Recently, a shortened Dscam (sDscam) gene family with tandemly arrayed 5′ cassettes in Chelicerata species has been identified, which encodes ∼50–100 isoforms. Chelicerata sDscams could be classified into two subfamilies, sDscamα and sDscamβ, containing one and two variable Ig domains, respectively. Crystal structures and cell aggregation assays demonstrated that both α and β subfamilies of sDscam used Ig1 for the isoform-specific trans recognition in a hand-in-hand manner. Furthermore, the cis interactions were established by the three FNIII domains of sDscam, which assemble into a cross fold with a kink between FNIII2 and FNIII3.

The crystal structures of sDscam Ig1 from both M. martensii and L. polyphemus revealed a common assembly of antiparallel homodimer for both α and β subfamilies of sDscam. More interestingly, in some Ig1 crystal structures (M. martensii α1, α7, and L. polyphemus α7), the two protomers within a homodimer were related via a 2-fold symmetry axis, namely, these two protomers had identical conformations. This implied that the homophilic trans interactions of Ig1 were also symmetry-related. Similarly, sDscam Ig1 also employs the ABED face to form an antiparallel homodimer. However, among the seven Ig1 structures reported here, the complementary electrostatic potential surface pattern (negative in one end, neutral in the middle, and positive in the other end) has been only observed in the three β isoforms, but not in any one of the four α isoforms. Moreover, all the Ig1 isoforms without exception have a potential N-linked glycosylation site (NXS/T) located at the F strand. This glycosylation prevents the CFG face from establishing homophilic interactions and helps define the interface of the sDscam homodimer.

>[2x]STVPQIKPFYFSTTLQEKQREQITCLAIAGDPPLSFSWTKDGINIDKFSDIIVETPKNFYSVLVILSIQPNHIGNYTCIVKNSVGSDSFTASLILKVP5-[(1R,3S)-3-aminocyclohexyl]-6-bromo-3-(1-methyl-1H-pyrazol-4-yl)pyrazolo[1,5-a]pyrimidin-7-amine 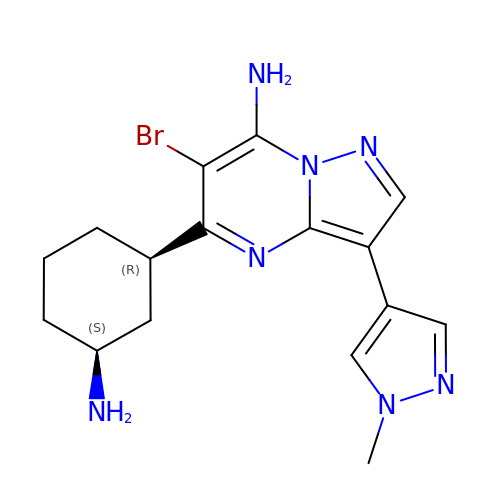| C16 H20 Br N7 | CKLKHZYNDIKOOE-KOLCDFICSA-N>[4x]SPYSSDTTPCCFAYIARPLPRAHIKEYFYTSGKCS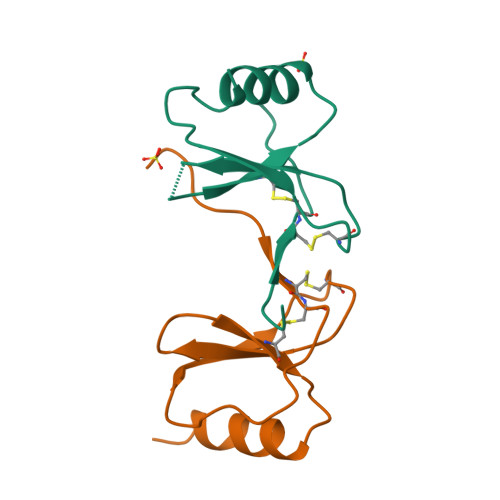NPAVVFVTAANAQVCANPEKKWVREYINSLEMS> MDPQGDAAQKTDTSHHDQDHPTFNKITPNLAEFAFSLYRQLAHQSNSTNILFSPVSIAAAFAMLSLGAKGDTHDEILEGLNFNLTEIPEAQIHEGFQELLRTLNQPDSQLQLTTGNGLFLSEGLKLVDKFLEDVKKLYHSEAFTVNFGDTEEAKKQINDYVEKGTQGKIVDLVKELDRDTVFALVNYIFFKGKWERPFEVKDTEEEDFHVDQVTTVKVPMMKRLGMFNIQHSKKLSSWVLLMKYLGNATAIFFLPDEGKLQHLENELTHDIITKFLENEDRRSASLHLPKLSITGTYDLKSVLGQLGITKVFSNGADLSGVTEEAPLKLSKAVHKAVLTIDEKGTEAAGAMFLEAIPRSIPPEVKFNKPFVFLIIEQNTKAPLFMGRVVNPTQK;> FIFLALLGAAVAFPVDDDDKIVGGYTCGANTVPYQVSLNSGYHFCGGSLINSQWVVSAAHCYKSGIQVRLGEDNINVVEGNEQFISASK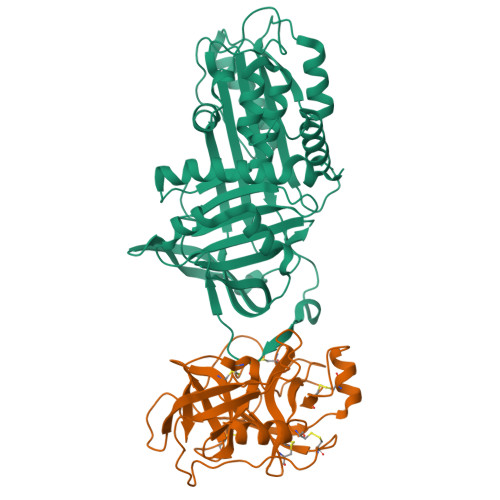SIVHPSYNSNTLNNDIMLIKLKSAASLNSRVASISLPTSCASAGTQCLISGWGNTKSSGTSYPDVLKCLKAPILSDSSCKSAYPGQITSNMFCAGYLEGGKDSCQGDAGGPVVCSGKLQGIVSWGSGCAQKNKPGVYTKVCNYVSWIKQTIASN>GHMQMPGIENIPATLSHGGRFIQYNIFGNIFEVTAKYKPPIMPIGKGAYGIVCSAMNSETNESVAIKKIANAFDNKIDAKRTLREIKLLRHMDHENIVAIRDIIPPPLRNAFNDVYIAYELMDTDLHQIIRSNQALSEEHCQYFLYQILRGLKYIHSANVLHRDLKPSNLLLNANCDLKICDFGLARVTSESDFMTEYVVTRWYRAPELLLNSSDYTAAIDVWSVGCIFMELMDRKPLFPGRDHVHQLRLLMELIGTPSEEELEFLNENAKRY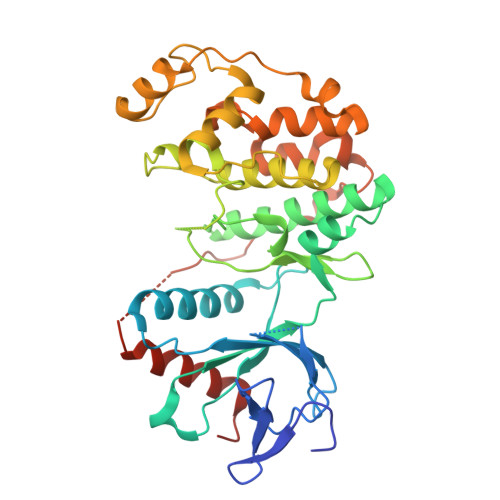IRQLPPYPRQSITDKFPTVHPLAIDLIEKMLTFDPRRRITVLDALAHPYLNSLHDISDEPECTIPFNFDFENHALSEEQMKELIYREALAFNPEYQQ[2x]octadecylphosphonic acid | 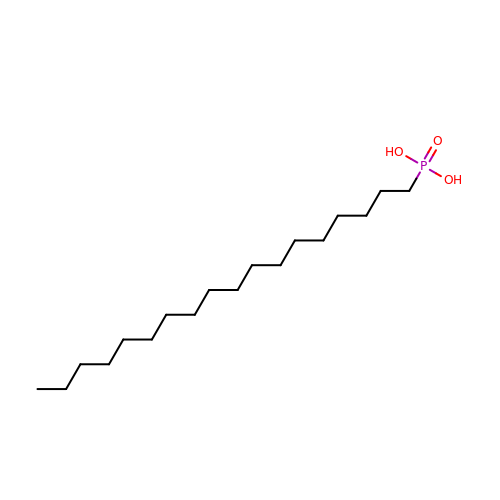C18 H39 O3 P | FTMKAMVLFVRZQX-UHFFFAOYSA-N>[2x]RTFDLEEKLQTNKYNANFVTFMEGKDFNVEYIQRGGLRDPLIFKNSDGLGIKMPDPDFTVNDVKMCV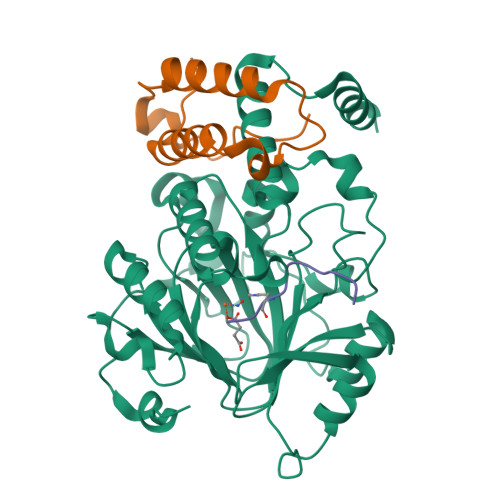GSRRMVDVMDVNTQKGIEMTMAQWTRYYETPEEEREKLYNVISLEFSHTRLENMVQRPSTVDFIDWVDNMWPRHLKESQTESTNAILEMQYPKVQKYCLMSVRGCYTDFHVDFGGTSVWYHIHQGGKVFWLIPPTAHNLELYENWLLSGKQGDIFLGDRVSDCQRIELKQGYTFVIPSGWIHAVYTPTDTLVFGGNFLHSFNIPMQLKIYSIEDRTRVPNKFRYPFYYEMCWYVLERYVYCITNRSHLTKDFQKESLSMDME;>QVHLTHFELEGLRCLVDKLESLPLHKKCVPTGIEDEDALIADVKILLEELASSDPKLALTGVPIVQWP[2x];>APATGGVKKPHRYRP[2x]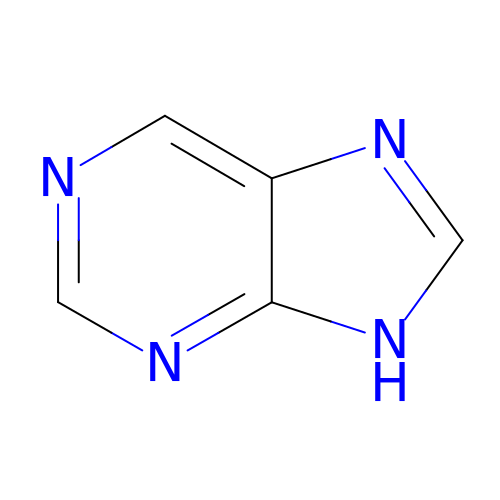9~{H}-purine | C5 H4 N4 | KDCGOANMDULRCW-UHFFFAOYSA-N> 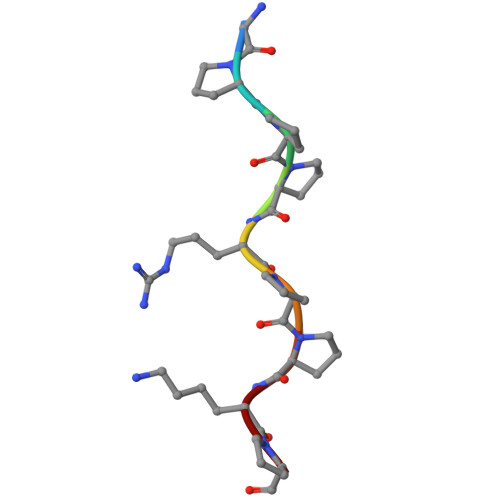APPPRPPKP> 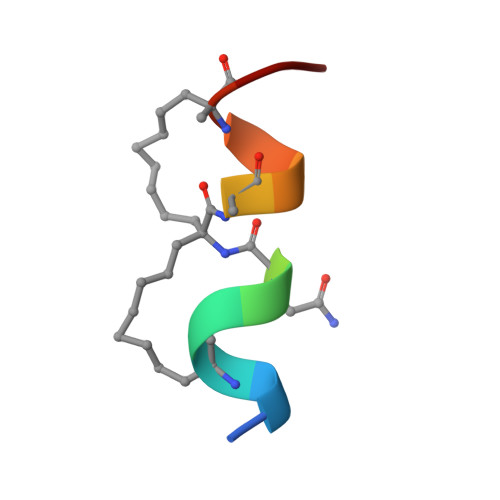NQLRAQXALQXVN> MKINIRDSTMVRPATETPITNLWNSNVDLVIPRFH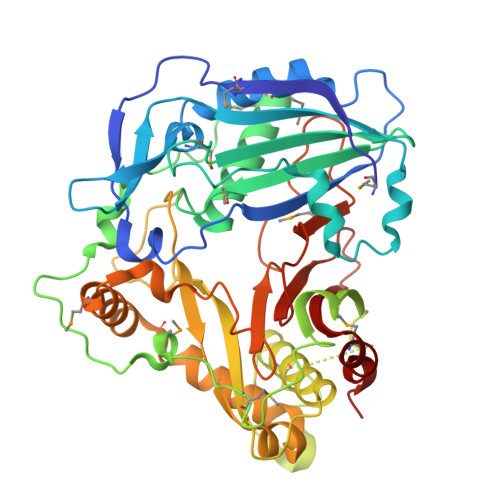TPSVYFYRPTGASNFFDPQVMKEALSKALVPFYPMAGRLKRDDDGRIEIDCNGAGVLFVVADTPSVIDDFGDFAPTLNLRQLIPEVDHSTGIHSFPLLVLQVTFFKCGGASLGVGMQHHAADGFSGLHFINTWSDMARGLDLTIPPFIDRTLLRARDPPQPAFHHVEYQPAPSMKIPLDPSKSGPENTTVSIFKLTRDQLVALKAKSKEDGNTVSYSSYEMLAGHVWRSVGKARGLPNDQETKLYIATDGRSRLRPQLPPGYFGNVIFTATPLAVAGDLLSKPTWYAAGQIHDFLVRMDDNYLRSALDYLEMQPDLSALVRGAHTYKCPNLGITSWVRLPIYDADFGWGRPIFMGPGGIPYEGLSFVLPSPTNDGSLSVAIALQSEHMKLFEKFLFEI The three human TFFs (TFF1, TFF2, and TFF3)1 are ubiquitous in mucosal environments. The trefoil domain is comprised of three loops (foils) formed by three disulfide bonds. TFF1 and TFF3 are disulfide-linked homo-dimers with each monomer possessing a single trefoil domain, while TFF2 is a single-chain protein with two trefoil domains. Using a combination of ELISA, isothermal titration calorimetry (ITC) and tryptophan quenching assays, we demonstrate that the cognate ligand for all TFFs is the GlcNAc-α-1,4-Gal disaccharide.

Initial attempts to co-crystallise the TFFs and their cognate ligand were confounded by the exceptional solubility of these proteins. Eventually we obtained mTFF1 crystals, though they only yielded an apo structure. An alignment of all mammalian TFF sequences revealed that all TFF1 proteins utilise a disaccharide-binding Asn, while all TFF3 proteins retain an Asp. TFF1 operates in the low pH gastric mucosa, while TFF3 does not, which suggested that a ligand-binding Asn or Asp may impact the pH profile of the lectin activity. At pH 2.6, the Kd for mTFF1 increased only slightly to 67 ± 1 µM, while for mTFF3 the Kd was 350 ± 60 µM; six-fold higher than at pH 7.4. The structure also provides insights into how TFF1 might bind H. pylori in an α-glucosidase sensitive manner. The core oligosaccharide of many H. pylori strains bears a Glc-α-1,4-Gal-branch, while the N-acetyl group of GlcNAc-α-1,4-Gal bound to the TFFs is solvent exposed and makes no interactions with the peptide. Clearly, the Glc-α-1,4-Gal branch of H. pylori core glycans could be easily accommodated in the TFF binding site.

>[3x]QTETCTVAPRERQNCGFPGVTPSQCANKGCCFDDTVRGVPWCFYPNTILEK>MAETDGSIPLIPVRMLNEHVYCPRLAYLMWVQGEFSHNEFTVDGVIRHRRVDAGGGVLPSETQEDSRIHARSVSLSSERLGITAKIDLVEGEGAYVSPVDYKRGKRPHVAGGAYEPERVQLCAQGLLLREHGFASDGGALYFVASRERVPVAFDDELIGRTLAAIDEMGRTALSGTMPPPLEDSPKCPRCSLVGICLPDEVRFLSHLSVEPRPIIPADGRGLPLYVQSPKAYVRKDGDCLVIEEERVRVAEARLGETSQVALFGNATLTTAALHECLRREIPVTWLSYGGWFMGHTVSTGHRNVETRTYQYQRSFDPETCLNLARRWIVAKIANCRTLLRRNWRGEGDEAKAPPGLLMSLQDDMRHAMRAPSLEVLLGIEGASAGRYFQHFSRMLRGGDGEGMGFDFTTRNRRPPKDPVNALLSFAYAMLTREWTVALAAVGLDPYRGFYHQPRFGRPALALDMMEPFRPLIADSTVLMAINNGEIRTGDFVRSAGGCNLTDSARKRFIAGFERRMEQEVTHPIFKYTISYRRLLEVQARLLTRYLSGEIPAYPNFVTR[4x];>[2x]MEHLYIVSYDIRNQRRWRRLFKTMHGFGCWLQLSVFQCRLDR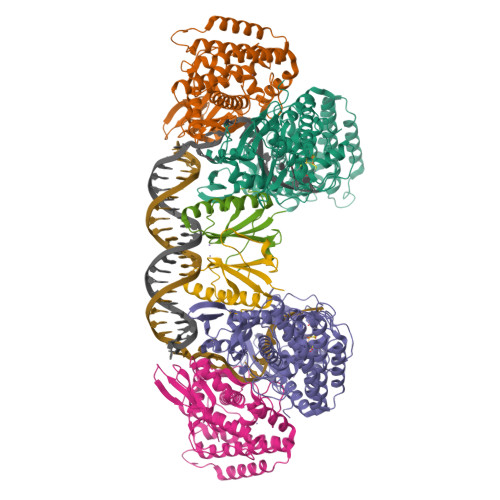IRIIKMEAAINEIVNHAEDHVLILDLGPAENVKPKVSSIGKTFDPILRQAVIV> MEPPAIPHITEGFYPLPEIVETFSHHVLQELVSLAEVLPSMSNVEKKKKILDWLLRSRAFTMRLLVLARWVHLSPSVHRCIDVVAFLQGQKFCFQNLVHVLQDIRYQLSFARLRNSDLVTALDILSTGTSLRLANAPTSKLYMLSESPLSTKQILQTLHALNMLIRIRLSLYEIIPTPFQHFTIANGRCTFTVPNEFSVSLTTNSQDPKSTGISFQWIVVDFQFHLPDFSSTPAKYRVFIELHLNEEIAAAFVLQKPILPLIYNILHKFCLYQRLNLLSQQTFQLSRE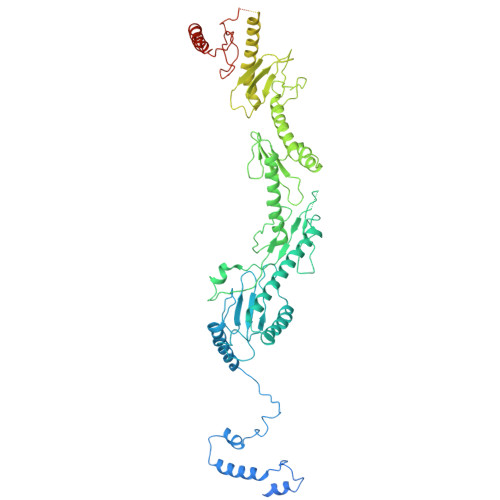SWLGHLRGVYDEKPPRLRLYYWPQLNVKKEGKPGKIGHYIHIFVNTQPISAFERTLSSKRSSCEYDHFLLLVEWHHDGIVEHVPLDDHMDAQHLLLLITQKHAQLILEQIRKELHPNIFSEHVGGGLKIHVFDNEIIVKVNSVTGRLVLSSSASPLSPPRHLRAAEKNIALNTQPPAQILNRLYFFCIQTQLLEVAQCAELHAVQGYYSFPYLTFSKGKWRKDGDSLWVLAYNVESNSWSVRLLNAAGQTLYTQDVHTTKGTLSIESFSRLSYLLEVQILLFNVQTACQARGMPFEYLPIPPKALIEDDFTTYVQTGCLCIMMPSSNEDMLPVVFVRAHDGQLIFDSRIKGKLPYQSETETEKNCYIDWRTGRITIRVQNFSSFEKTWIGLLKLVALSKTSAFNVDCITLKHVDFTYLDDEKFRATIHDDNTFTLHFFNRHSPFHLISQFLQDTFSDGPSAIQPLRVIMDRTRGVLVAQELGYVVLARSLRQYRIILSKNHGIQVLLNRHGCILQDLSYLSADSRYLEGTQTLTSQWEPCSWLNTVWEGDLGDDELNGQIEAAPEMHLIKMNKTADLTAILKRILAISRKKXXXXXXXXXXXXXXXXXXXXXXXXXXXXXXXXXXXXXXXXXXXXXXXXXXXX> KFIYGDVDGNGSVRINDAVLIRDYVLGKINEFPYEYGM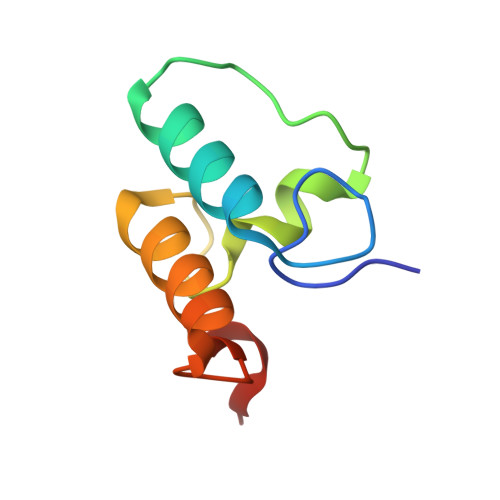LAADVDGNGSIKSIDAVLVRDYVLGKIFLFPVEEKEE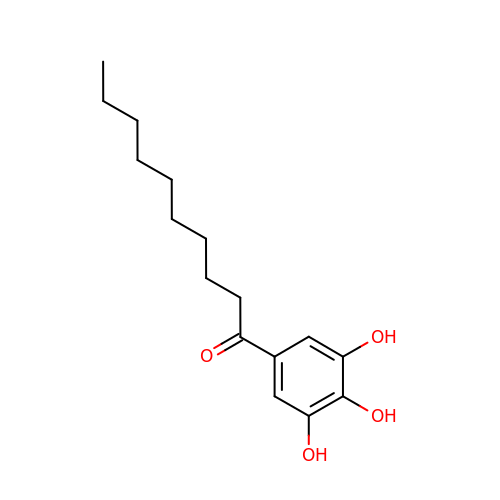1-(3,4,5-trihydroxyphenyl)decan-1-one | C16 H24 O4 | HZQGIOUWWQWGCZ-UHFFFAOYSA-N>[2x]MATVEPETTPTPNPPTTEEEKTESNQEVANPEHYIKHPLQNRWALWFFKNDKSKTWQANLRLISKFDTVEDFWALYNHIQLSSNLMPGCDYSLFKDGIEPMWEDEKN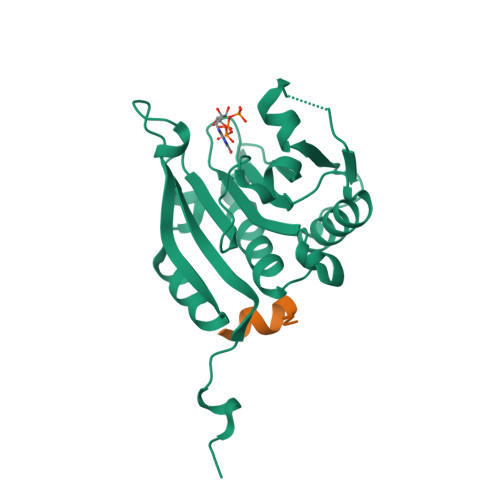KRGGRWLITLNKQQRRSDLDRFWLETLLCLIGESFDDYSDDVCGAVVNVRAKGDKIAIWTTECENREAVTHIGRVYKERLGLPPKIVIGYQSHADTATKSGSTTKNRFVV;>XKKRYSREFLLGFX[2x]> GSHMMRSPYEYHHDLGMNYTLIRDELIVGSQPQKPEDIDHLKQEQNVAYILNLQQDKDIEYWGIDLDSIVRRCKELGIRHMRRPAKDFDPLSLRSQLPKAVSSLEWAVSEGKGRVYVHSSAGLGRAPGVSIAYMYWFCDMNLNTAYDTLVSKRPCGPNKGAIRGATYDLAKNDPWKEPFESLPENAFEDIADWERKLIQERV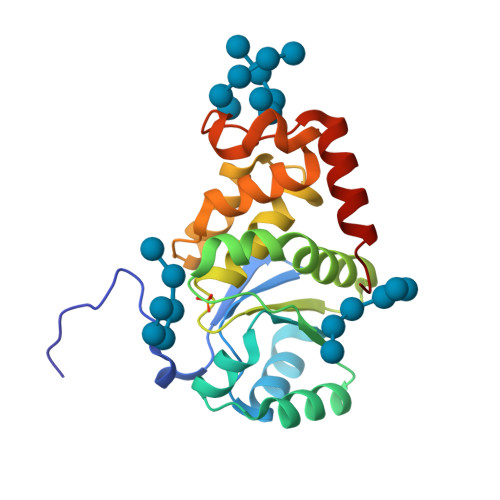RALRGT B. bacteriovorus is an obligate bacterial predator of other Gram-negative bacteria, exploiting adaptations that allow consumption from inside the prey cell periplasm. The DgcB protein appends the C-terminal GGDEF enzymatic domain with an N-terminal forkhead-associated (FHA) domain, known to be used (in other proteins) for interactions with phosphopeptide ligands. DgcB comprised a ~30aa tail, 100aa FHA, 20aa linker and 160aa GGDEF domain. We provide the molecular basis for initiation of c-di-GMP production, demonstrating that the stimulus is a phosphopeptide tail present on the DgcB GGDEF synthase itself.

To resolve this issue, we obtained 1.87 Å data on a new crystal form (tail-FHA only, lacking the GGDEF domain) comprised of residues 1–135 of DgcB. In this new form, four FHA domains comprise the asymmetric unit, with each monomer arranged at ~90˚ to the neighboring domain. Upon imposing crystal symmetry, it is apparent that each monomer contacts a symmetry-related molecule in precisely the same manner as chains A and B of the full-length DgcB structure (mediated through D56). Hence it can be inferred that the FHA:FHA contacts in full-length DgcB are not dictated by constraints imposed by the GGDEF domain. For one of the FHA domains, difference density was observable at the putative phosphopeptide-binding cleft (next to consensus residues S75, R76 and T96). Our high resolution data allowed us to unambiguously model this density as residues K13-S19 of the previously disordered N-terminal tail of DgcB. It was not possible to assign the tail as originating from a specific chain (chain B, C and D FHA domains are all close enough to span the distance to the bound tail). In agreement with assignment of the FHA domain as a putative phosphothreonine receptor, the interactions between the tail and FHA cleft centre around residue T14, which is conserved in homologues of DgcB. The FHA cleft makes three hydrogen bonds to the tail (involving R61, T96 and N97), which binds in a linear conformation across the apical face of the FHA fold. Aligning the N-terminal tail from a representative group of DgcB homologues reveals a pattern of conservation across a seven residue span (−3 to +3 with respect to the central threonine); our structure underlines the importance of the +3 position (V17), which points downward into the cleft and is a crucial recognition feature of the peptide substrate in other FHA-based sensory systems.

> KTSIVAS;>VPPAIVVLIGPPGYVGKQYPITASDIVIGRSVESQVYIDDKSLSRSHAKFAVNGSEVSVIDLGSTNKTIVNGQVIPPLASCLLKNNDQIKTGNVIFKFLEKGSIE[4x]> SNAPEPDMITIFIGTWNMGNAPPPKKITSWFLSKGQGKTRDDSADYIPHDIYVIGTQEDPLGEKEWLELLRHSLQEVTSMTFKTVAIHTLWNIRIVVLAKPEHENRISHICTDNVKTGIANTLGNKGAVGVSFMFNGTSLGFVNSHLTSGSEKKLRRNQNYMNILRFLALGDKKLSPFNITHRFTHLFWLGDLNYRVELPTWEAEAIIQKIKQQQYSDLLAHDQLLLERKDQKVF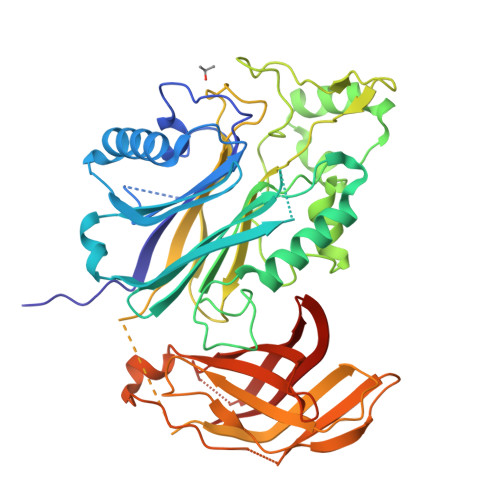LHFEEEEITFAPTYRFERLTRDKYAYTKQKATGMKYNLPSWCDRVLWKSYPLVHVVCQSYGSTSDIMTSDHSPVFATFEAGVTSQFVSKNGPGTVDSQGQIEFLACYATLKTKSQTKFYLEFHSSCLESFVKSQEGANAAGSEGELVVRFGETLPKLKPIISDPEYLLDQHILISIKSSDSDESYGEGCIALRLETTEAQHPIYTPLTHHGEMTGHFRGEIKLQTSQG>MGSDKIHHHHHHMKIDILDKGFVELVDVMGNDLSAVRAARVSFDMGLKDEERDRHLIEYLMKHGHETPFEHIVFTFHVKAPIFVARQWFRHRIASYNELSGRYSKLSYEFYIPSPERLEGYKTTIPPERVTEKISEIVDKAYRTYLELIESGVPRRVARIVLPLNLYTRFFWTVNARSLMNFLNLRADSHAQWEIQQYALAIARIFKEKCPWTFEAFLKYAYKGDILKEVQV[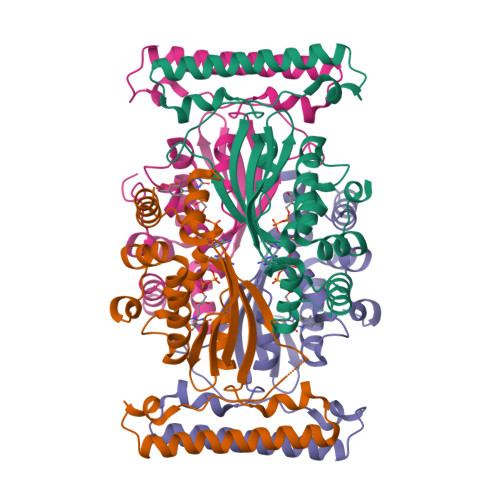4x]>MDLVEEILRLKEERNAIILAHNYQLPEVQDIADFIGDSLELARRATRVDADVIVFAGVDFMAETAKILNPDKVVLIPSREATCAMANMLKVEHILEAKRKYPNAPVVLYVNSTAEAKAYADVTVTSANAVEVVKKLDSDVVIFGPDKNLAHYVAKMTGKKIIPVPSKG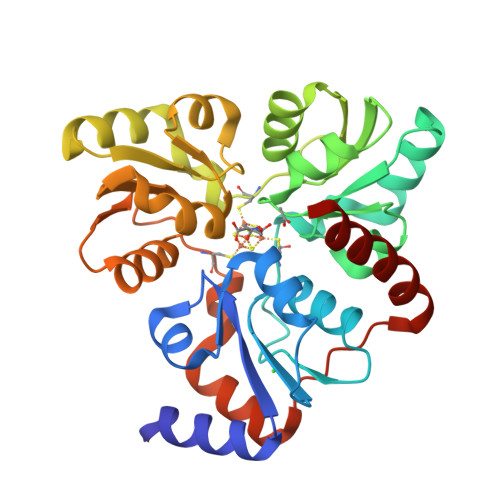HCYVHQKFTLDDVERAKKLHPNAKLMIHPQCIPEVQEKADIIASTGGMIKRACEWDEWVVFTEREMVYRLRKLYPQKKFYPAREDAFCIGMKAITLKNIYESLKDMKYKVEVPEEIARKARKAIERMLEMSK[2x]>[4x]GSMPGFLTAFEYSEKRKMVFHITTGSQEFDKLLGGGIESMAITEAFGEFRTGKTQLSHTLCVTAQLPGAGGYPGGKIIFIDTENTFRPDRLRDIADRFNVDHDAVLDNVLYARAYTSEHQMELLDYVAAKFHEEAGIFKLLIIDSIMALFRVDFSGRGELAERQQKLAQMLSRLQKISEEYNVAVFVTNQMTADPGATMTFQADPKKPIGGHILAHASTT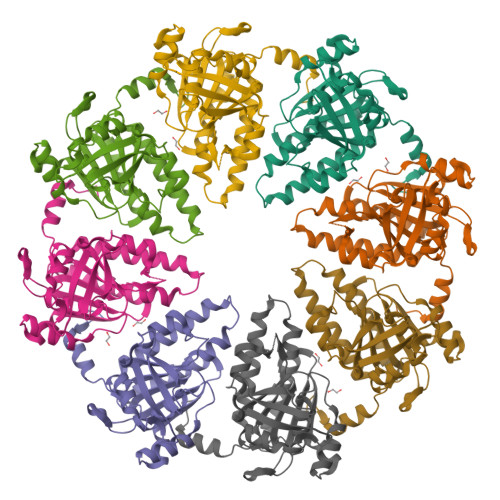RISLRKGRGELRIAKIYDSPEMPENEATFAITAGGIGDAKE Here, we demonstrate that the centriolar protein SAS-6 forms rod-shaped homodimers that interact through their N-terminal domains to form oligomers. Proteins of the SAS-6 family comprise an N-terminal domain with the evolutionarily conserved PISA motif, followed by a segment with a predicted coiled coil and a less-conserved C-terminal region predicted to be disordered. Furthermore and in conclusion, because these residues are well conserved among SAS-6 orthologs, we propose that the self-assembly of SAS-6 homodimers into a 9-fold symmetric ring structure is a fundamental property at the root of the universal 9-fold symmetry of centrioles.

By contrast, we were able to produce soluble recombinant proteins from C. reinhardtii Bld12p (Nakazawa et al., 2007), which has the same domain organization as other SAS-6 orthologues. Like for C. elegans SAS-6, we started by producing a fragment encompassing the N-terminal domain (denoted crN) and solved its structure to 2.1 Å resolution by X-ray crystallography. We found that the asymmetric unit of the crystal contained three equivalent crN dimers (denoted the crN-dimer hereafter). The monomers in each dimer are related by local 2-fold symmetry. The overall structure and organization of the crN-dimer, as well as the F145 residue engaged at the N-N interface and corresponding to I154 of C. elegans SAS-6, are similar to that of the C. elegans ceN-dimer. The stability of the crN-dimer in solution was assessed by ITC, and the Kd was determined to be 60 ± 20 μM, which is similar to that of the ceN-dimer from C. elegans. Overall, these results indicate that there is strong structural conservation among N-terminal domains of SAS-6 proteins across evolution. In addition, they demonstrate that the function of the critical residue within the β6-β7 loop mediating the interaction between pairs of N-terminal domains is likewise conserved. Having the structures of both the crN-dimer and the crCC-dimer of Bld12p allowed us to build a structural model of higher-order oligomers using both dimer interfaces. Strikingly, when crCC-dimers were associated such that their N-terminal domains interact as observed in the crN-dimer, we obtained a ring with a 9-fold symmetry (see Experimental Procedures for full description of the modeling).

>[6x]GSMPLLLDDGDPKAQTGFDLSTATTLFWRPVPVHVKQQDREDVLEELTFRILTGVAKQNHNLRILRIHISSDSDLFFLHTLEVSEEDFQSLKNDQGILVDFASFPGKIISLLEKCILAQPGDSPRFQAVLTIRGGESVFKIVEINDFKQLPHITLAFRPGN> GSCEKENIGIEVTPVNAKFIITPVVIDATTGTDVTQSAEISFSKGNGTYEGTPELASESININAKYKGMTGSASVTIPALKAGQFGAKEVTIILSEN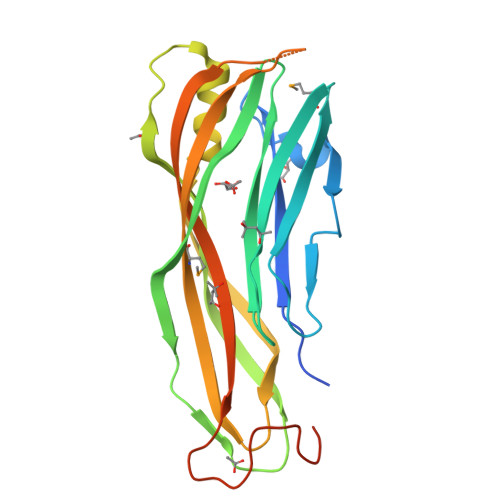FFAQEESSNSQIETTKHSGFKNNTSDYWYYITVTYTKKEGSEVIKNDYEGDDSEIKNIIDAYNKGVREDKVTLNDVQVLAHSRFSVFVDYMKTTSVYQIIEKSPKRDGNPVASFTVDSYNTIVSPKNEQIPGHGHAPSHGHGHGHGDDSNAGGGIIIAD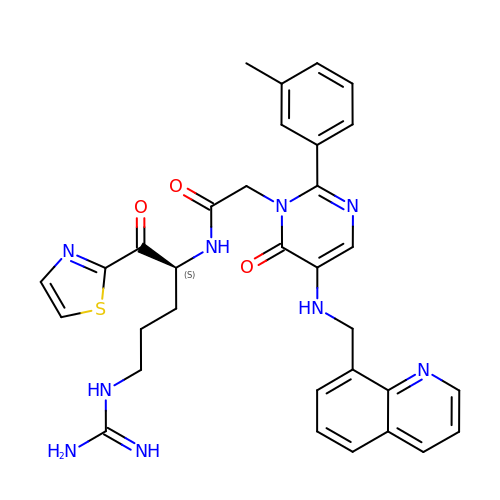N-[4-GUANIDINO-1-(THIAZOLE-2-CARBONYL)-BUTYL]-2-{6-OXO-5-[(QUINOLIN-8-YLMETHYL)-AMINO]-2-M-TOLYL-6H-PYRIMIDIN-1-YL}-ACETAMIDE | C32 H33 N9 O3 S | BWWLNFRQHXSLCW-DEOSSOPVSA-N>MDQKPQPAKTHATEV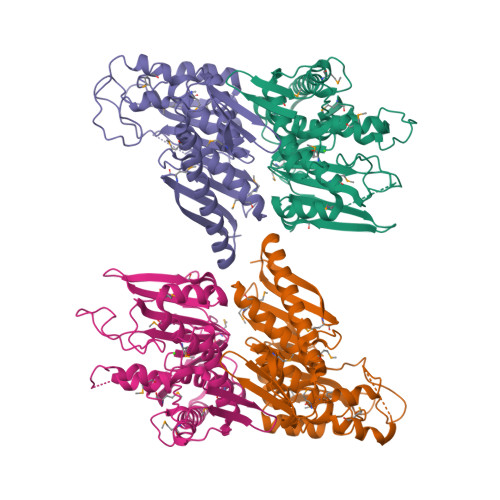TVLEGKTMGTFWRASIPGIDAKRSAELKEKIQTQLDADDQLLSTYKKDSALMRFNDSQSLSPWPVSEAMADIVTTSLRIGAKTDGAMDITVGPLVNLWGFGPEQQPVQIPSQEQIDAMKAKTGLQHLTVINQSHQQYLQKDLPDLYVDLSTVGEGYAADHLARLMEQEGISRYLVSVGGALNSRGMNGEGLPWRVAIQKPTDKENAVQAVVDINGHGISTSGSYRNYYELDGKRLSHVIDPQTGRPIEHNLVSVTVIAPTALEADAWDTGLMVLGPEKAKEVVRREGLAVYMITKEGDSFKTWMSPQFKSFLVSEKNLEHHHHHH[4x]> MSLTTSHFIPFPREMVWDWHTRKGAVARLTPPFIPLNPITQAERLADGTTIFSLPAGLKWVARHDLSGFLNGSRFTDVCLTAPVKALANWRHVHNFVDQDGGTLITDSVSTRLPASTLTGMFAYRQTQLIEDLKFLSRTSTLFDGSPLTVAITGSRGLVGRALTAQLQTGGHEVIQLVRKEPKPGKRFWDPLNPASDLLDGADVLVHLAGEPIFGRFNDSHKEAIRESRVLPTKFLAE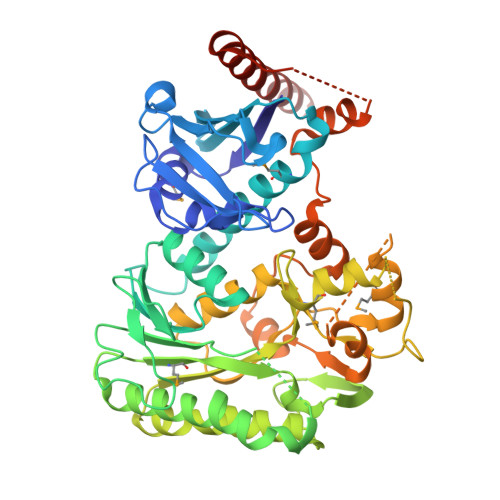LVAESTQCTTMISASAVGFYGHDRGDEILTEESESGDDFLAEVCRDWEHATAPASDAGKRVAFIRTGVALSGRGGMLPLLKTLFSTGLGGKFGDGTSWFSWIAIDDLTDIYYRAIVDAQISGPINAVAPNPVSNADMTKILATSMHRPAFIQIPSLGPKILLGSQGAEELALASQRTAPAALENLSHTFRYTDIGAAIAHELGYEQLADFAQQQEIEAERKQERAELKAAKKIAKKAPVLEESPTNLEDPEEVEQSILSSILNFRRKRNDLEHHHHHH>[2x]SNAMILIDGKSLSKDLKERLATQVQEYKHHTAITPKLVAIIVGNDPASKTYVASKEKACAQVGIDSQVITLPEHTTESELLELIDQLNNDSSVHAILVQLPLPAHINKNNVIY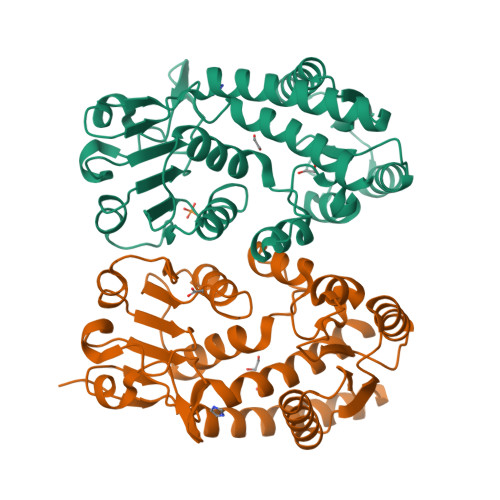SIKPEKDVDGFHPTNVGRLQLRDKKCLESCTPKGIMTMLREYGIKTEGAYAVVVGASNVVGKPVSQLLLNAKATVTTCHRFTTDLKSHTTKADILIVAVGKPNFITADMVKEGAVVIDVGINHVDGKIVGDVDFAAVKDKVAAITPVPGGVGPMTITELLYNTFQCAQELNR>MAHHHHHHMSRPINPDVVNRPLVICGPSGTGKSTLLKTLFESQPNTFGFSVSHTTRKPRPGEENGREYHFVTKEEFMEGVGKGEFLEWAEFGGNCYGTTFAALTALHPRRCILDIELQGVLQLKAKAPLQTPPLEPVFLFLSPPSISQLKSRLSGRGTET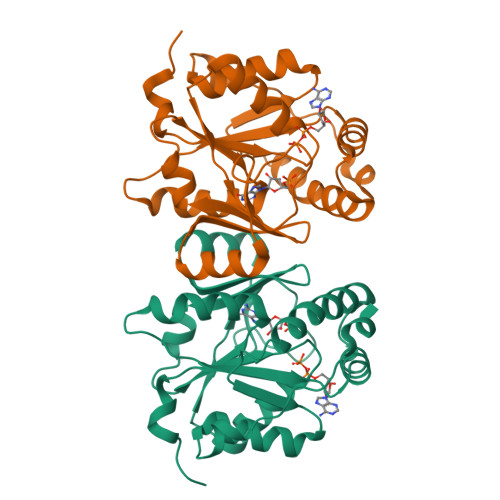DASIRKRLDAAKEELRYAKEGKYDVYVVNDDLKVAGEKLEKVAMGWEGWKTCGDTLPELNLAELD[4x]>[2x]MGSHHHHHHMGQSVEVEILLNDAESRKRAEHKTEDGKKEKYFLFYDGETVSGKVSLSLKNPNKRLEHQGIKIEFIGQIELYYDRGNHHEFVSLVKDLARPGEITQSQAFDFEFTHVEKPYESYTGQN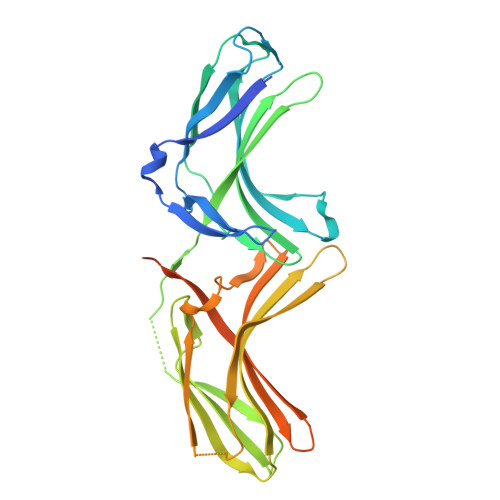VKLRYFLRATISRRLNDVVKEMDIVVHTLSTYPELNSSIKMEVGIEDCLHIEFEYNKSKYHLKDVIVGKIYFLSVEIKIKHMEIDIIKRETTGTGPNVYHENDTIAKYEIMDGAPVRGESIPIRLFLAGYELTPTMRDINKKFSVRYYLNLVLIDEEERRYFKQQEVVLWRKGDIVRKSMSHQAAIASQRFEGTTSLGEVRTPGQLSDNNSRQ>MQLTPREVEKLMIYTLSDVAFKRKARGLKLNYPEAVSIITVTAMEGARDGKSVEDVMKEASKVLTKDDVMDGVADLIPNVQVEAIFTDGSRLVTVHDPIK[4x];>[4x]MSTKTNSTKATSEKTDSLKTNSGTKSSAGYSEQNTPLGGCILADTPITFNENKPVTKVKVRNTGDRPIQVGSHFHFFEVNRALEFDRAAAYGKRLNISSTTAIRFEPGDETEVPLIPFGGKQTLYGFNNLVDGWTGEGVVPNSERPDKLEAIRRAAERGFKSSK;>[4x]MPQISRQEYAGLFGPTTGDKIRLGDTNLFIEIEKDLRGYGEESVYGGGKSLRDGMGANNHLTRD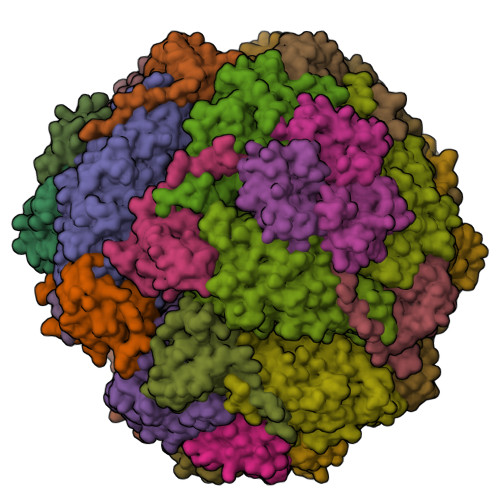NGVLDLVITNVTIVDARLGVIKADVGIRDGKIAGIGKSGNPGVMDGVTPGLVVGVSTDAISGEHLILTAAGIDTHIHLISPQQAYHALSNGVATFFGGGIGPTDGTNGTTVTPGPWNIRQMLRSVEGLPVNVGILGKGNSYGRGPLLEQAIAGVVGYKVHEDWGATANALRHSLRMADEMDIQVSVHTDSLNECGYVEDTIDAFEGRTIHTFHTEGAGGGHAPDIIRVASQPNVLPSSTNPTLPYGVNSQAELFDMIMVCHNLNPNVPADVSFAESRVRPETIAAENVLHDMGVISMFSSDSQAMGRVGENWLRVMQTANAMKASRGKLPEDAPGNDNFRVLRYVAKITINPAIAQGVSHVIGSVEVGKMADLVLWDPRFFGAKPKMVIKGGMINWAAMGDPNASLPTPQPVFYRPMFGAMGKTMQDTCVTFVSQAALDDGVKEKAGLDRQVIAVKNCRTISKHDLVRNDQTPNIEVDPETFAVKVDGVHATCEPIDTAAMNQRYFFG Using a combination of biochemistry and cryo–electron microscopy, we characterized the first enzyme of the transsulfuration pathway, cystathionine β-synthase (MtbCbs) in Mtb. We demonstrated that MtbCbs is a heme-less, pyridoxal-5′-phosphate–containing enzyme, allosterically activated by S-adenosylmethionine (SAM). The rectangular-shaped 3D structure of the tetrameric MtbCbs contains an N-terminal catalytic core region (7 to 296 residues), C-terminal Bateman module (329 to 464 residues), and a connecting linker between the catalytic core and the Bateman module (297 to 328 residues). In this study, we resolved the full-length structure of MtbCbs in its native, activated, and substrate-bound conformations.

Single-particle cryo-EM was used to analyze the conformation of the native tetrameric MtbCbs. The Bateman module is composed of two CBS motifs, CBS1 (T329-E397) and CBS2 (A403-E459), existing in tandem repeats. The density of the connecting linker is well ordered and stable in our cryo-EM structure, which suggests the absence of any disordered amino acid residues. We propose that the oligomerization of MtbCbs requires initial association of the monomers via their core domains to create dimers, which subsequently associate via their respective Bateman modules to yield the tetrameric assembly. The 3D structure indicates that the dimerization and tetramerization interfaces are stabilized predominantly by hydrophobic interactions. The active site lysine, K44, is located inside the catalytic core domain on helix α4 and forms a Schiff base interaction with PLP. In native MtbCbs, the active site K44 is buried inside the core region by a flexible loop (G40, G41, S42, S43, D45, and R46), making K44 relatively inaccessible to the substrates. In the absence of Ser, a stable continuous density is present in the cryo-EM map between K44 and PLP at an RMSD value of 6σ. This indicates the formation of internal aldimine at the active site.

>[4x]MARIAQHISELIGGTPLVRLNSVVPDGAGTVAAKVEYLNPGGSSKDRIAVKMIEAAEASGQLKPGGTIVEPTSGNTGVGLALVAQRRGYKCVFVCPDKVSEDKRNVLIAYGAEVVVCPTAVPPHDPASYYSVSDRLVRDIDGAWKPDQYANPEGPASHYVTTGPEIWADTEGKVTHFVAGIGTGGTITGAGRYLKEVSGGRVRIVGADPEGSVYSGGAGRPYLVEGVGEDFWPAAYDPSVPDEIIAVSDSDSFDMTRRLAREEAMLVGGSCGMAVVAALKVAEEAGPDALIVVLLPDGGRGYMSKIFNDAWMSSYGFLRSRLDGSTEQSTVGDVLRRKSGALPALVHTHPSETVRDAIGILREYGVSQMPVVGAEPPVMAGEVAGSVSERELLSAVFEGRAKLADAVSAHMSPPLRMIGAGELVSAAGKALRDWDALMVVEEGKPVGVITRYDLLGFLSEGAGRRKLAAALEHHHHHH> MTSVTRSEIIDEKGPVMSKTHDHQLESSLSPVEVFAKTSASLEMNQGVSEERIHLGSSPKKGGNCDLSHQERLQSKSLHLSPQEQSASYQDRRQSWRRASMKETNRRKSLHPIHQGITELSRSISVDLAESKRLGCLLLSSFQFSIQKLEPFLRDTKGFSLESFRAKASSLSEELKHFADGLETDGTLQKCFEDSNGKASDFSLEASVAEMKEYITKFSLERQTWDQLLLHYQQEAKEILSRGSTEAKITEVKVEPMTYLGSSQNEVLNTKPDYQKILQNQSKVFDCMELVMDELQGSVKQLQAFMDESTQCFQKVSVQLGKRSMQQLDPSPARKLLKLQLQNPPAIHGSGSGSCQ;> MAAFRDIEEVSQGLLSLLGANRAEAQQRRLLGRHEQVVERLLETQDGAEKQLREILTMEKEVAQSLLNAKEQVHQGGVELQQLEAGLQEAGEEDTRLKASLLQLTRELEELKEIEADLERQEKEVDEDTTVTIPSAVYVAQLYHQVSKIEWDYECEPGMVKGIHHGPSVAQPIHLDSTQLSRKFISDYLWSLVDTEW;> MVEDELALFDKSINEFWNKFKSTDTSCQMAGLRDTYKDSIKAFAEKLSVKLKEEERMVEMFLEYQNQISRQNKLIQEKKDNLLKLIAEVKGKKQELEVLTANIQDLKEEYSRKKETISTANKANAERLKRLQKSADLYKDRLGLEIRKIYGEKLQFIFTNIDPKNPESPFMFSLHLNEARDYEVSDSAPHLEGLAEFQENVRKTNNFSAFLANVRKAFTATVYN;> MDGVSSEANEENDNIERPVRRRHSSILKPPRSPLQDLRGGNERVQESNALRNKKNSRRVSFADTIKVFQTESHMKIVRKSEMEGCSAMVPSQLQLLPPGFKRFSCLSLPETETGENLLLIQNKKLEDNYCEITGMNTLLSAPIHTQMQQKEFSIIEHTRERKHANDQTVIFSDENQMDLTSSHTVMITKGLLDNPISEKSTKIDTTSFLANLKLHTEDSRMKKEVNFSVDQNTSSENKIDFNDFIKRLKTGKCSAFPDVPDKENFEIPIYSKEPNSASSTHQMHVSLKEDENNSNITRLFREKDDGMNFTQCHTANIQTLIPTSSETNSRESKGNDITIYGNDFMDLTFNHTLQILPATGNFSEIENQTQNAMDVTTGYGTKASGNKTVFKSKQNTAFQDLSINSADKIHITRSHIMGAETHIVSQTCNQDARILAMTPESIYSNPSIQGCKTVFYSSCNDAMEMTKCLSNMREEKNLLKHDSNYAKMYCNPDAMSSLTEKTIYSGEENMDITKSHTVAIDNQIFKQDQSNVQIAAAPTPEKEMMLQNLMTTSEDGKMNVNCNSVPHVSKERIQQSLSNPLSISLTDRKTELLSGENMDLTESHTSNLGSQVPLAAYNLAPESTSESHSQSKSSSDECEEITKSRNEPFQRSDIIAKNSLTDTWNKDKDWVLKILPYLDKDSPQSADCNQEIATSHNIVYCGGVLDKQITNRNTVSWEQSLFSTTKPLFSSGQFSMKNHDTAISSHTVKSVLGQNSKLAEPLRKSLSNPTPDYCHDKMIICSEEEQNMDLTKSHTVVIGFGPSELQELGKTNLEHTTGQLTTMNRQIAVKVEKCGKSPIEKSGVLKSNCIMDVLEDESVQKPKFPKEKQNVKIWGRKSVGGPKIDKTIVFSEDDKNDMDITKSYTIEINHRPLLEKRDCHLVPLAGTSETILYTCRQDDMEITRSHTTALECKTVSPDEITTRPMDKTVVFVDNHVELEMTESHTVFIDYQEKERTDRPNFELSQRKSLGTPTVICTPTEESVFFPGNGESDRLVANDSQLTPLEEWSNNRGPVEVADNMELSKSATCKNIKDVQSPGFLNEPLSSKSQRRKSLKLKNDKTIVFSENHKNDMDITQSCMVEIDNESALEDKEDFHLAGASKTILYSCGQDDMEITRSHTTALECKTLLPNEIAIRPMDKTVLFTDNYSDLEVTDSHTVFIDCQATEKILEENPKFGIGKGKNLGVSFPKDNSCVQEIAEKQALAVGNKIVLHTEQKQQLFAATNRTTNEIIKFHSAAMDEKVIGKVVDQACTLEKAQVESCQLNNRDRRNVDFTSSHATAVCGSSDNYSCLPNVISCTDNLEGSAMLLCDKDEEKANYCPVQNDLAYANDFASEYYLESEGQPLSAPCPLLEKEEVIQTSTKGQLDCVITLHKDQDLIKDPRNLLANQTLVYSQDLGEMTKLNSKRVSFKLPKDQMKVYVDDIYVIPQPHFSTDQPPLPKKGQSSINKEEVILSKAGNKSLNIIENSSAPICENKPKILNSEEWFAAACKKELKENIQTTNYNTALDFHSNSDVTKQVIQTHVNAGEAPDPVITSNVPCFHSIKPNLNNLNGKTGEFLAFQTVHLPPLPEQLLELGNKAHNDMHIVQATEIHNINIISSNAKDSRDEENKKSHNGAETTSLPPKTVFKDKVRRCSLGIFLPRLPNKRNCSVTGIDDLEQIPADTTDINHLETQPVSSKDSGIGSVAGKLNLSPSQYINEENLPVYPDEINSSDSINIETEEKALIETYQKEISPYENKMGKTCNSQKRTWVQEEEDIHKEKKIRKNEIKFSDTTQDREIFDHHTEEDIDKSANSVLIKNLSRTPSSCSSSLDSIKADGTSLDFSTYRSSQMESQFLRDTICEESLREKLQDGRITIREFFILLQVHILIQKPRQSNLPGNFTVNTPPTPEDLMLSQYVYRPKIQIYREDCEARRQKIEELKLSASNQDKLLVDINKNLWEKMRHCSDKELKAFGIYLNKIKSCFTKMTKVFTHQGKVALYGKLVQSAQNEREKLQIKIDEMDKILKKIDNCLTEMETETKNLEDEEKNNPVEEWDSEMRAAEKELEQLKTEEEELQRNLLELEVQKEQTLAQIDFMQKQRNRTEELLDQLSLSEWDVVEWSDDQAVFTFVYDTIQLTITFEESVVGFPFLDKRYRKIVDVNFQSLLDEDQAPPSSLLVHKLIFQYVEEKESWKKTCTTQHQLPKMLEEFSLVVHHCRLLGEEIEYLKRWGPNYNLMNIDINNNELRLLFSSSAAFAKFEITLFLSAYYPSVPLPSTIQNHVGNTSQDDIATILSKVPLENNYLKNVVKQIYQDLFQDCHFYH;> MSVDPMTYEAQFFGFTPQTCMLRIYIAFQDYLFEVMQAVEQVILKKLDGIPDCDISPVQIRKCTEKFLCFMKGHFDNLFSKMEQLFLQLILRIPSNILLPEDKCKETPYSEEDFQHLQKEIEQLQEKYKTELCTKQALLAELEEQKIVQAKLKQTLTFFDELHNVGRDHGTSDFRESLVSLVQNSRKLQNIRDNVEKESKRLKIS;> MAGSPELVVLDPPWDKELAAGTESQALVSATPREDFRVRCTSKRAVTEMLQLCGRFVQKLGDALPEEIREPALRDAQWTFESAVQENISINGQAWQEASDNCFMDSDIKVLEDQFDEIIVDIATKRKQYPRKILECVIKTIKAKQEILKQYHPVVHPLDLKYDPDPAPHMENLKCRGETVAKEISEAMKSLPALIEQGEGFSQVLRMQPVIHLQRIHQEVFSSCHRKPDAKPENFITQIETTPTETASRKTSDMVLKRKQTKDCPQRKWYPLRPKKINLDT;> MAEASSANLGSGCEEKRHEGSSSESVPPGTTISRVKLLDTMVDTFLQKLVAAGSYQRFTDCYKCFYQLQPAMTQQIYDKFIAQLQTSIREEISDIKEEGNLEAVLNALDKIVEEGKVRKEPAWRPSGIPEKDLHSVMAPYFLQQRDTL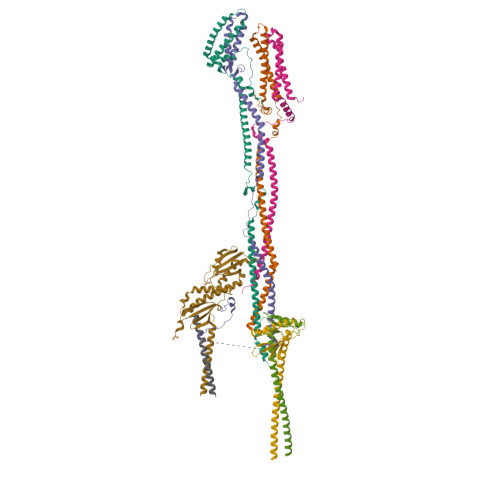RRHVQKQEAENQQLADAVLAGRRQVEELQLQVQAQQQAWQALHREQRELVAVLREPE;> MEAAETEAEAAALEVLAEVAGILEPVGLQEEAELPAKILVEFVVDSQKKDKLLCSQLQVADFLQNILAQEDTAKGLDPLASEDTSRQKAIAAKEQWKELKATYREHVEAIKIGLTKALTQMEEAQRKRTQLREAFEQLQAKKQMAMEKRRAVQNQWQLQQEKHLQHLAEVSAEVRERKTGTQQELDRVFQKLGNLKQQAEQERDKLQRYQTFLQLLYTLQGKLLFPEAEAEAENLPDDKPQQPTRPQEQSTGDTMGRDPGVSFKAVGLQPAGDVNLP>SNVRATYTVIFKNASGLPNGYDNWGWGCTLSYYGGAMIINPQEGKYGAVSLKRNSGSFRGGSLRFDMKNEGKVKILVENSEADEKFEVETISPSDEYVTYILDVDFDLPFDAIDFQDAPGNGDRIWIKNLVHSTGSADDFVDP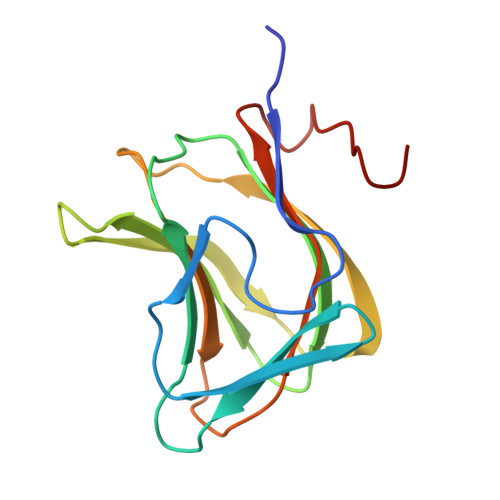INLHHH[2x]> S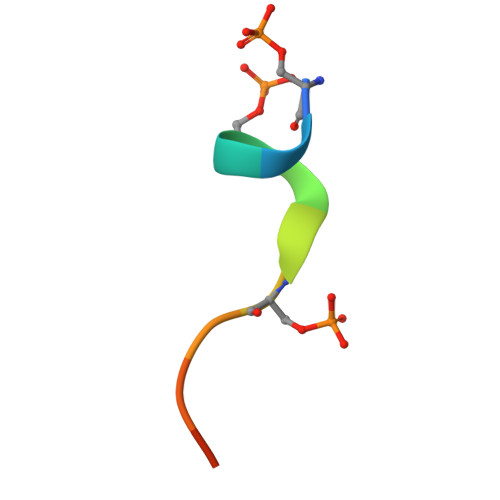SASTVSVGSSY>MSLWRQTPDLEQLNASQKNSIGDLLGIRFEAFDDESLTASMPVDSRTHQPFGLLHGGASVVLAASLGSMASYLCVDTSQYYCVGLEVNANHLRGLRSGRVTAVARAIHLGRTTHVWDI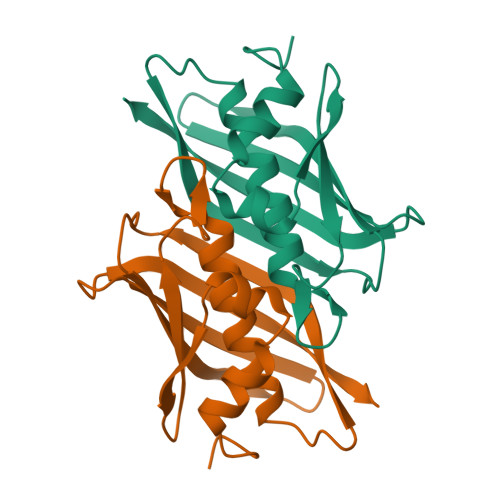RLSGDDGKPSCIARLTMAVVPLAGRALEHHHHHH[6x]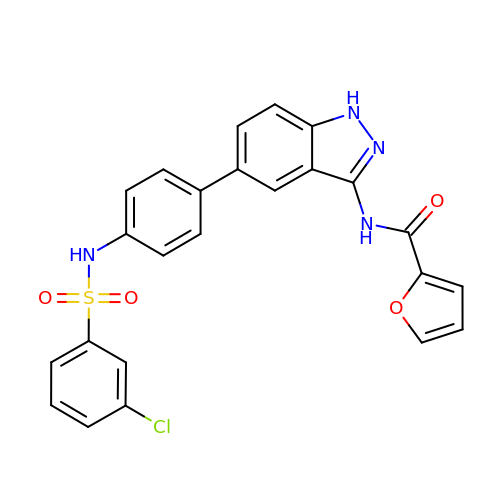N-[5-(4-{[(3-chlorophenyl)sulfonyl]amino}phenyl)-1H-indazol-3-yl]furan-2-carboxamide | C24 H17 Cl N4 O4 S | LBIIPAPYSBCHHH-UHFFFAOYSA-N> MGKIFEDNSLTIGHTPLVRLNRIGNGRILAKVESRNPSFSVKCRIGANMIWDAEKRGVLKPGVELVEPTSGNTGIALAYVAAARGYKLTLTMPETMSIERRKLLKALGANLVLTEGAKGMKGAIQKAEEIVASNPEKYLLLQQFSNPANPEIHEKTTGPEIWEDTDGQVDVFIAGVGTGGTLTGVSRYIKGTKGK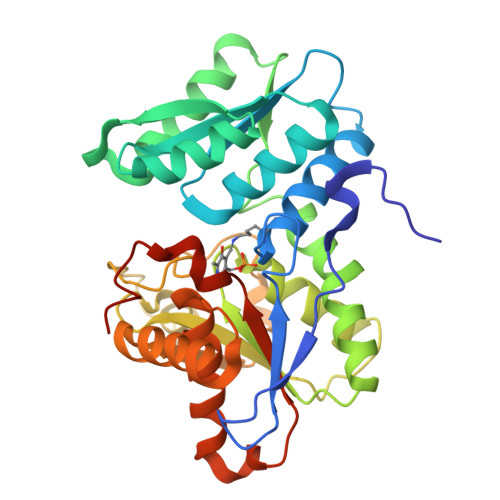TDLISVAVEPTDSPVIAQALAGEEIKPGPHKIQGIGAGFIPANLDLKLVDKVIGITNEEAISTARRLMEEEGILAGISSGAAVAAALKLQEDESFTNKNIVVILPSSGERYLSTALFADLFTEKELQQ> PAREFQRDLLDWFARERRDLPWRKDRDPYKVWVSEVMLQQTRVETVIPYFEQFIDRFPTLEALADADEDEVLKAWEGLGYYSRVRNLHAAVKEVKTRYGGKVPDDPDEFSRLKGVGPYTVGAVLSLAYGVPEPAVDGNVMRVLSRLFLVTDDIAKCSTRKRFEQIVREIMA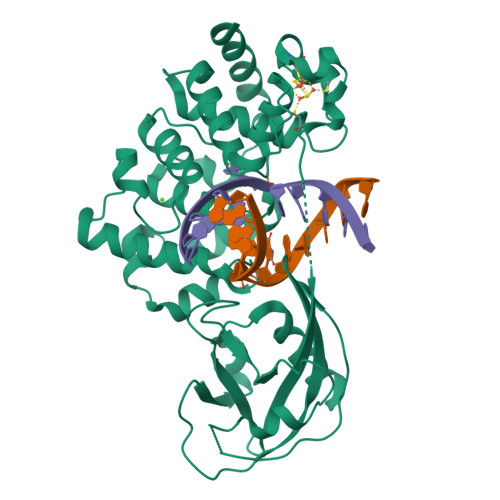YENPGAFNEALIELGALVCTPRRPSCLLCPVQAYCQAFAEGVAEELPVKMKKTAVKQVPLAVAVLADDEGRVLIRKRDSTGLLANLWEFPSCETDGADGKEKLEQMVGEQYGLQVELTEPIVSFEHAFSHLVWQLTVFPGRLVHGGPVEEPYRLAPEDELKAYAFPVSHQRVWREYKEWAS> MTSRINKPWRISHSPNSKIPSPVREKLNRLSRNQDVFPILDLQELVICLQSCDFALATQENISRPTSDYMVTLYKQIIENFMGISVESLLNSSNQETGDGHLQEENENIYLDTLNVLVLNKICFKFFENIGVQDFNMTDLYKPEAQRTQRLLSAVVNYARFREERMFDCNSFILQMESLLGQINKLNDEIKQLQKDFEVEVKEIEAAYSLLSGHI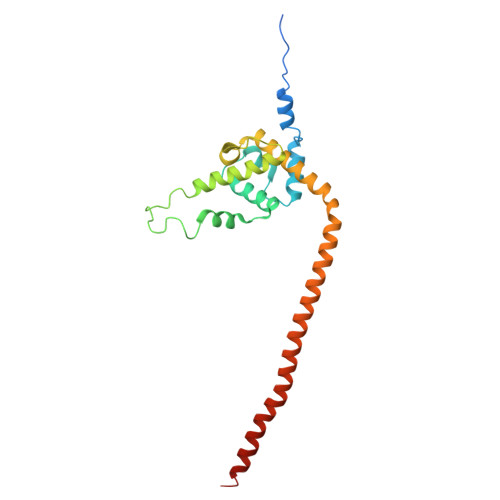NKYMNEMLEYMQ>[6x]MGSLNTEDVLENSSAFGVTNPLDPEEFRRQGHMIIDFLADYYRDVEKYPVRSQVEPGYLRKRLPETAPYNPESIETILQDVTTEIIPGLTHWQSPNYYAYFPSSGSVAGFLGEMLSTGFNVVGFNWMSSPAATELESVVMDWFGKMLNLPESFLFSGSGGGVLQGTSCEAILCTLTAARDRKLNKIGREHIGRLVVYGSDQTHCALQKAAQVAGINPKNFRAIKTFKENSFGLSAATLREVILEDIEAGLIPLFVCPTVGTTSSTAVDPISPICEVAKEYEMWVHVDAAYAGSACICPEFRHFIDGVEEADSFSLNAHKWFFTTLDCCCLWVKDPSALVKALSTNPEYLRNKATESRQVVDY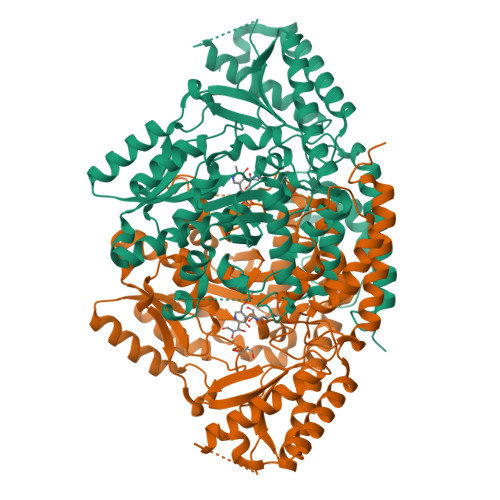KDWQIALSRRFRSLKLWMVLRSYGVTNLRNFLRSHVKMAKTFEGLICMDGRFEITVPRTFAMVCFRLLPPKTIKVYDNGVHQNGNGVVPLRDENENLVLANKLNQVYLETVNATGSVYMTHAVVGGVYMIRFAVGSTLTEERHVIYAWKILQEHADLILGKFSEADFSS4-(1H-imidazol-5-yl)pyridine | C8 H7 N3 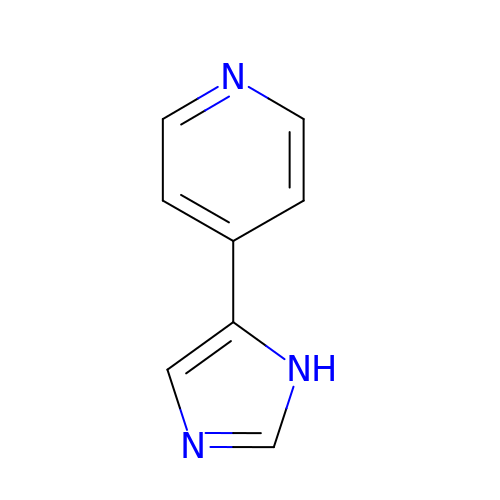| AJQQGJNKKDEODG-UHFFFAOYSA-N>IPDGVVSALSLRERIREHLSSEESVGLLFSGCTGINDKTLGARGGEVIMVTSGSGMGKSTFVRQQALQWGTAMGKKV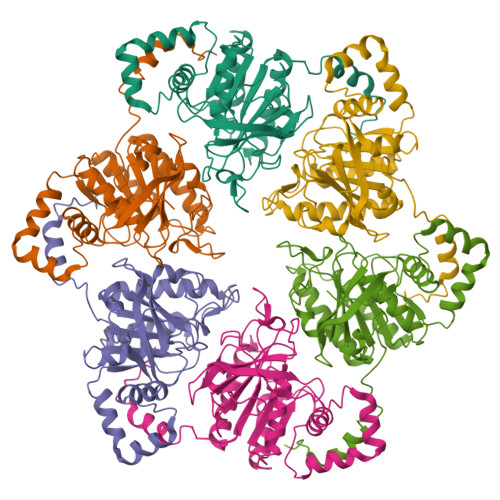GLAMLEESVEETAEDLIGLHNRVRLRQSDSLKREIIENGKFDQWFDELFGNDTFHLYDSFAEAETDRLLAKLAYMRSGLGCDVIILDHISIVVSASGESDERKMIDNLMTKLKGFAKSTGVVLVVICHLKNPDKGKAHEEGRPVSITDLRGSGALRQLSDTIIALERNQQGDMPNLVLVRILKCRFTGDTGIAGYMEYNKETGWLEPSSYSG[6x]> MESKRNKPGKATGKGKPVGDKWLDDAGKDSGAPIPDRIADKLRDKEFK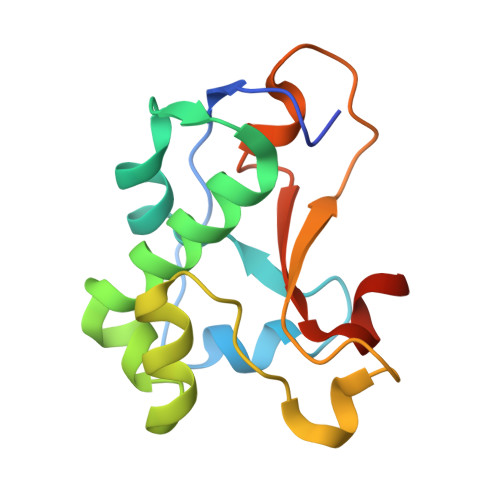NFDDFRKKFWKEVAKDPDLAKQFSKANQRNIKDGNAPFARESDQVGGRTTYELHHDKPISQDGGVYDMNNIRVTTPKRAIDIHRGK The O-GlcNAc modified protein can be transformed back into its native state by O-GlcNAc hydrolysis by O-GlcNAcase (OGA). Two bacterial apparent OGA orthologues from Clostridium perfringens and Bacteroides thetaiotaomicron have been studied by protein crystallography to obtain insight in the active site and the catalytic mechanism. Recent kinetic and structural data obtained from hOGA and bacterial homologues (GH84 family members) have revealed that GH84 and GH20 perform hydrolysis via substrate-assisted catalysis and the active site architecture is structurally conserved. In order to identify new human O-GlcNAcase inhibitors, a high-throughput screening assay was performed based on the release of 4-methylumbelliferol (4MU) from the pseudo substrate 4MU-GlcNAc, initially using the bacterial OGA homologue from C. perfringens (CpOGA) which has recently been shown to be a good model of hOGA.

To determine the binding mode of the competitive OGA inhibitors, these compounds were soaked into CpOGA crystals. Ordered electron density could only be obtained for diprophylline. The electron density for the inhibitor was located in the active site of CpOGA, where it competes with substrate binding, in agreement with the competitive inhibition mode determined from kinetic studies. Diprophylline interacts with three active site residues via hydrogen bonds. The 2-OH and 3-OH hydroxyl groups from the 2,3-dihydroxypropyl moiety hydrogen bond to the carboxyl group of residue Asp401, which is conserved between bacterial (CpOGA) and hOGA. This interaction mimics the interaction of GlcNAc 4/6-OH with Asp401. The xanthine moiety is sandwiched between the two aromatic residues Trp394 and Tyr335, where it participates in π-stacking interactions. Furthermore, Lys218 and Asn396 hydrogen bond to the N9 and O6 atoms from the theophylline moiety, respectively. The electron density unambiguously represented the S-enantiomer of diprophylline. Interestingly, the loop carrying the catalytic acid Asp298 and Asp297 is in the ‘open’ conformation.

>[2x]VGPKTGEENQVLVPNLNPTPENLEVVGDGFKITSSINLVGEEEADENAVNALREFLTANNIEINSENDPNSTTLIIGEVDDDIPELDEALNGTTAENLKEEGYALVSNDGKIAIEGKDGDGTFYGVQTFKQLVKESNIPEVNITDYPTVSARGIVEGFYGTPWTHQDRLDQIKFYGENKLNTYIYAPKDDPYHREKWREPYPESEMQRMQELINASAENKVDFVFGISPGIDIRFDGDAGEEDFNHLITKAESLYDMGVRSFAIYWDDIQDKSAAKHAQVLNRFNEEFVKAKGDVKPLITVPTEYDTGAMVSNGQPRAYTRIFAETVDPSIEVMWTGPGVVTNEIPLSDAQLISGIYNRNMAVWWNYPVTDYFKGKLALGPMHGLDKGLNQYVDFFTVNPMEHAELSKISIHTAADYSWNMDNYDYDKAWNRAIDMLYGDLAEDMKVFANHSTRMDNKTWAKSGREDAPELRAKMDELWNKLSSKEDASALIEELYGEFARMEEACNNLKANLPEVALEECSRQLDELITLAQGDKASLDMIVAQLNEDTEAYESAKEIAQNKLNTALSSFAVISEKVAQSFIQEALSFDLTLI>[8x]MTRLFMLVCLGIVCQGTTGNILRGESLNKSLPILHEWKFFDYDFGSDERRQDAILSGEYDYKNNYPSDIDQWHDKIFVTMLRYNGVPSSLNVISKKVGDGGPLLQPYPDWSFAKYDDCSGIVSASKLAIDKCDRLWVLDSGLVNNTQPMCSPKLLTFDLTTSQLLKQVEIPHDVAVNATTGKGRLSSLAVQSLDCNTNSDTMVYIADEKGEGLIVYHNSDDSFHRLTSNTFDYDPKFTKMTIDGESYTAQDGISGMALSPMTNNLYYSPVASTSLYYVNTEQFRTSDYQQNDIHYEGVQNILDTQSSAKVVSKSGVLFFGLVGDSALGCWNEHRTLERHNIRTVAQSDETLQMIASMKIKEALPHVPIFDRYINREYILVLSNKMQKMVNNDFNFDDVNFRIMNANVNELILNTRCENPDNDRTPFKISIHL;>[8x]MSKIVAVVVLAAFCVAMLVSDVS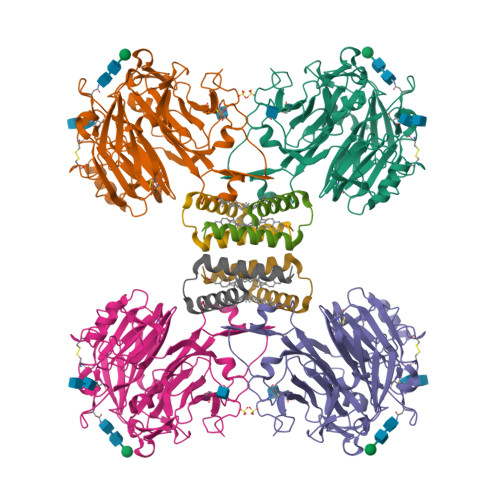AKTSISVKGESNVDVVSQINSLVSSIVSGANVSAVLLAQTLVNILQILIDANVFA Herein, a combination of genetic, biochemical and structural studies was used to demonstrate that MAB_4384 is part of the TetR family of regulators, which represses the transcriptional expression of the MmpS5/MmpL5 efflux pump. MAB_4384 belongs to the type I class TetR family of regulators, characterized by a divergent orientation to one of the adjacent target genes. The TetR transcriptional regulatory factors are common single component signal transduction systems found in bacteria. These proteins possess a conserved helix-turn-helix (HTH) signature at the N-terminal of the DNA-binding domain as well as a ligand binding domain (LBD) located at the C-terminal part. In contrast, the binding of a specific ligand to the LBD induces structural changes, conducting the dissociation of the repressor from the target DNA, and the subsequent transcription of the TetR-regulated genes.

The crystal structure of the native protein was subsequently solved with the partial model obtained from the SAD data and refined to a resolution of 1.9 Å. The asymmetric unit contains two subunits. Analysis of the crystal packing using the PISA server predicted the existence of a stable homodimer formed within the crystal, consistent with other TetR regulators and with the SEC profile of MAB_4384 in solution. The DBD is composed of three α-helices α1: residues 12–33, α2: 39–46, and α3: 50–56, where helices 2 and 3 form a helix-turn-helix (HTH) motif. The LBD is made of seven α-helices, α4: 60–82, α5: 88–104, α6: 107–114, α7: 121–143, α8: 155–170, α9: 178–188, and α10: 205–211. The surface of dimerization of about 1,700 Å2 is mediated by 31 residues mainly from helices α8 and α9 of each subunit and involves numerous interactions notably five salt bridges, fourteen hydrogen bonds and van der Waals interactions. Interestingly, we noticed the presence of extra electron density in the LBD of chain B in a rather hydrophobic pocket. Due to the occurrence of an extra electron density within the LBD of MAB_4384 and that the closest structure of MAB_4384 is LfrR in its ligand bound form, it is very likely that MAB_4384 was crystallized in its open conformation, i.e., its derepressed form that is not able to interact with DNA. Residues Arg55 from chains A and B are about 56 Å apart. From these results it can be inferred that the DBDs of MAB_4384 are too far from each other to bind to the DNA groove. These observations combined with the presence of an unidentified ligand in the LBD strongly suggest that the MAB_4384 structure is in an open conformation.

>[2x]GMNGREVAHRPLRKDAERNRKRVIAAARELFAVHGLESTLNEVAHHAGLGVGTVYRRFPTKEALFEAIYVDGMDQLSGLAEAALRHENSWEGFEWFVHQMCEITATNRGLREIAFSKAHGGDHVEAGRARLLPLLSKVVERAQEDGYLRPEASATDMPFFGVLTGAVSEFAGEVNADLWRRYMAILIEGMRRRDDQERLEVDALDEAQIDAAMTTWQPAGSG4-[(4-{[4-(4-cyano-2,6-dimethylphenoxy)-5-(pyridin-4-yl)pyrimidin-2-yl]amino}piperidin-1-yl)methyl]benzamide 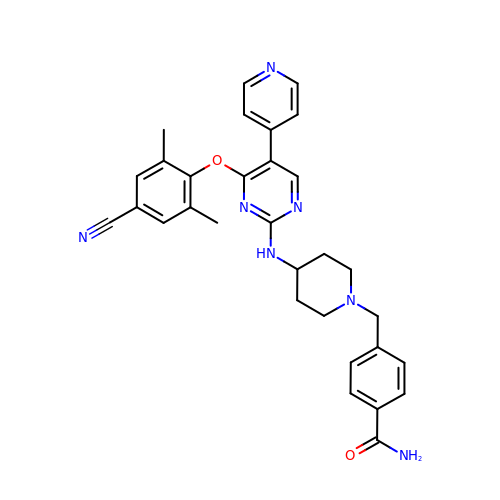| C31 H31 N7 O2 | VMVRZYRSNHFXGE-UHFFFAOYSA-N>[2x]MGNLTGNSKKAADSGDKPVIKMYQIGDKPDNLDELLANANKIIEEKVGAKLDIQYLGWGDYGKKMSVITSSGENYDIAFADNYIVNAQKGAYADLTELYKKEGKDLYKALDPAYIKGNTVNGKIYAVPVAANVASSQNFAFNGTLLAKYGIDISGVTSYETLEPVLKQIKEKAPDVVPFAIGKVFIPSDNFDYPVANGLPFVIDLEGDTTKVVNRYEVPRFKEHLKTLHKFYEAGYIPKDVATSDTSFDLQQDTWFVREETVGPADYGNSLLSRVANKDIQIKPITNFIKKNQTTQVANFVISNNSKNKEKSMEILNLLNTNPELLNGLVYGPEGKNWEKIEGKENRVRVLDGYKGNTHMGGWNTGNNWILYINENVTDQQIENSKKELAEAKESPALGFIFNTDNVKSEISAIANTMQQFDTAINTGTVDPDKAIPELMEKLKSEGAYEKVLNEMQKQYDEFLKNKKLEHHHHHH

The genome of S. pneumoniae contains genes that encode a suite of proteins that are biochemically capable of performing the various concerted steps needed to completely depolymerize and transport all classes of N-glycans found on host glycoconjugates. Here we characterize SpGH92 (TIGR4 locus tag SP_2145) as an α-mannosidase that trims the terminal α-(1,2)-linked mannose residues on high-mannose glycans to generate a substrate for EndoD. We also identify a solute binding protein (SBP; NgtS) from an ABC transporter (ABCNG) that binds soluble N-glycans and, through X-ray crystallography, reveal the molecular basis of its interaction with these branched glycans. The identification of an ABC transporter that possesses an SBP, NgtS, that is specific to the recognition of N-glycan fragments suggests that this is likely the convergence point of the complex and high mannose N-glycan processing sides of the N-glycan degradation pathway, with this transporter functioning to import soluble N-glycan fragments into the bacterium.

NgtS also bound to Man1GlcNAc; however, the low affinity and limited quantities of the sugar precluded binding analysis by ITC. Instead, we employed a UV difference binding analysis by taking advantage of a perturbation in the UV absorbance of the protein upon sugar binding. Used in a quantitative fashion we obtained an affinity constant of 1.2 (± 0.1) ×104 M−1 for Man1GlcNAc, and thus approximately two orders of magnitude lower than what was obtained for Man5GlcNAc. Despite these two complexes being obtained with different ligands and in different spacegroups, the overall conformations of NgtS were very similar (rmsd of 1.0 Å over 427 matched Cα positions); both complexes were in a “closed” conformation relative to the “open” conformation obtained in the absence of ligand. An overlay of the structures in complex with the two ligands showed that, within positional error of the structures, the location of Man1GlcNAc is the same as the corresponding Man1GlcNAc portion of Man5GlcNAc. The reducing end of the carbohydrate is oriented into the base of the protein binding cleft and fully sequestered from bulk solvent with no room for additional residues present at the reducing end, consistent with our proposal that NgtS specifically binds the products of EndoD hydrolysis (i.e. having only the single non-reducing GlcNAc residue). Only four direct hydrogen bonds are made between these two monosaccharide residues, though a notably extensive network of water-mediated hydrogen bonds is present. The recognition of this disaccharide motif is completed by the indole ring Trp386, which sits over the glycosidic bond and oriented parallel to the co-planar arrangement of the Man and GlcNAc pyranose rings such that the aromatic ring of Trp386 packs against the α-face of GlcNAc and the β-face of Man.> MGSSH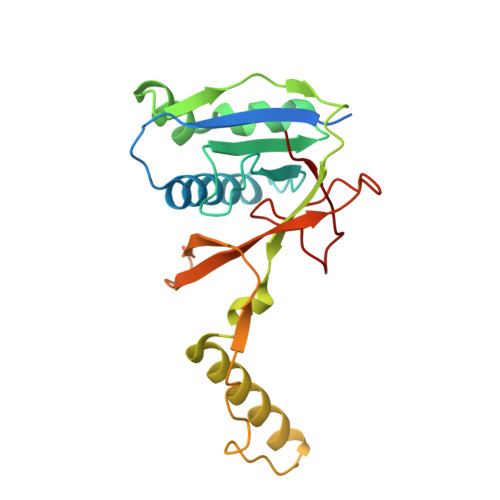HHHHHSQDPNSSMVKWYYKTITFLPELCNNESLAAKCLRVLHGFNYQYETRNIGVSFPLWCDATVGKKISFVSKNKIELDLLLKQHYFVQMEQLQYFHISNTVLVPEDCTYVSFRRCQSIDKLTAAGLARKIRRLEKRALSRGEQFDPSSFAQKEHTAIAHYHSLGESSKQTNRNFRLNIRMLSEQPREGNSIFSSYGLSNSENSFQPVPLI> GPMIDLYTAATPNGHKVSIALEEMGLPYTVHALSFDKKEQKAPEFLRINPNG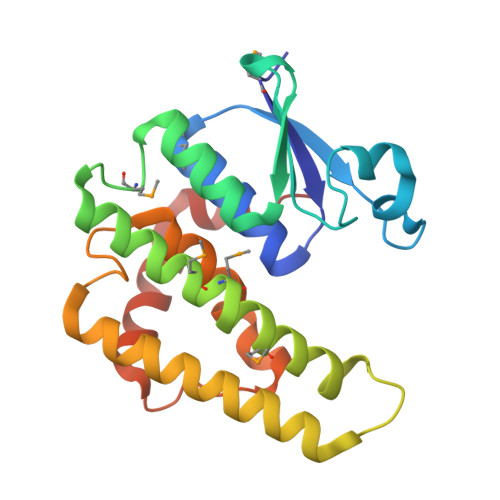RIPAIVDRSNDDFAVFESGAILVYLAEKTGQLMPTDVKGRSRVIQWLMFQMGGVGPMQGQANVFFRYFPEKLQGAIDRYQHETRRLYEVLDGRLGEAEYLAGDYSIADIATYPWVRIHDWSGVAVDGLDNLQRWIAALEARPAVQRGLLVPR Z-2-(3-bromophenyl) propanal oxime | C9 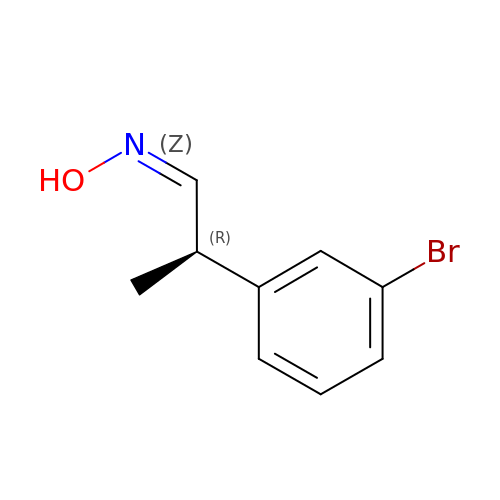H10 Br N O | SPBCOZIJYSLWMT-KSRYWAHESA-N>GQANHPTAAVVTEKQQMLEQHLQDVRKRVQDLEQKMKVVENLQDDFDFNYKTLKSQGDMQDLNGNNQSVTRQKMQQLEQMLTALDQMRRSIVSELAGLLSAMEYVQKTLTDEELADWKRRQQIACIGGPPNICLDRLENWITSLAESQLQTRQQIKKLEELQQKVSYKGDPIVQHRPMLEERIVELFRNLMKSAFVVERQPCMPMHPDRPLVIKTGVQFTTKVRLLVKFPELNYQLKIKVCIDKDSGDVAALRGSRKFNILGTNTKVMNMEESNNGSLSAEFKHLTLREQRCGNGGRANCDASLIVTEELHLITFETEVYHQGLKIDLETHSLP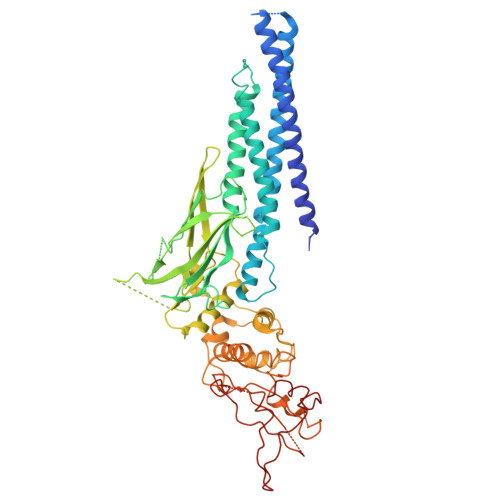VVVISNICQMPNAWASILWYNMLTNNPKNVNFFTKPPIGTWDQVAEVLSWQFSSTTKRGLSIEQLTTLAEKLLGPGVNYSGCQITWAKFCKENMAGKGFSFWVWLDNIIDLVKKYILALWNEGYIMGFISKERERAILSTKPPGTFLLRFSESSKEGGVTFTWVEKDISGKTQIQSVEPYTKQQLNNMSFAEIIMGYKIMDATNILVSPLVYLYPDIPKEEAFGKYCR[2x]>GPGSKPFTLPILTIGELSNSRFPAPIDELYTSPNEGLVVQPQNGRSTLDGELLGTTQLVPSNICSLRGRINAHLPDNQHRWNMQVTNANGTPFDPTEDVPAPLGTPDFLANIYGVTSQRNPDNTCRAHDGILATWSPKFTPKLGSVVLGTWEDRDFDINQPTRFTPVGLYDTDHFNQWALPNYSGALTLNMNLAPSVAPLFPGEQLLFFRSHIPLKGGTSNGAIDCLLPQEWVQHFYQESAPSSTDVALIRYTNPDTGRVLFEAKLHRQGFITVANSGSRPIVVPPNGYFRFDSWVNQFYSLAPM[2x]

The norovirus genome contains three open reading frames (ORF1 to 3), where ORF1 encodes the nonstructural proteins, ORF2 encodes the capsid protein (VP1), and ORF3 encodes a minor structural protein (VP2). The S domain forms a scaffold surrounding the viral RNA, whereas the P domain contains the determinants of strain diversity and recognition of attachment factors. There is considerable antigenic drift among human noroviruses, and new genetic variants evolve every other year, which can result in new epidemics worldwide. It is well known that human noroviruses bind with various specificities to histo-blood group antigens (HBGAs), which are present in saliva, on the surface of epithelial cells, and in mucosal secretions. To elucidate the constraints on non-HBGA binders from a structural perspective, we determined the X-ray crystal structures of the capsid-protruding domains (P domains) of two GII.1 (HV and noro485) nonbinders and one GII.2 (SMV) HBGA nonbinder.

HV was the first GII.1 virus detected in 1977 (15), noro485 (GII.1) was discovered in ~2005 (16), and SMV (GII.2) was identified in 1982 (17). HV, noro485, and SMV P domains diffracted to 1.86, 1.50, and 1.60 Å resolutions, respectively. The equivalent residues in the HV P domain were Cys345, Arg346, Asp375, and Gly438; in noro485, they were Cys345, Arg346, Asp375, and Gly438; and in SMV, they were Asn352, Arg353, Asp382, and Gly445. In the noro485 and SMV structures, Asp375 and Asp382, respectively, were pointing ~180° away from the fucose, whereas in the HV structure, Asp375 was missing because of the lack of electron density. Additionally, in the noro485 P domain structure, the polypeptide backbone of the loop hosting Asp375 (termed loop A) superimposed poorly onto the corresponding GII. Moreover, a neighboring loop (termed loop B) may have influenced the orientation and stability of loop A. For example, in noro485, loop B was oriented differently from that of GII. However, our new data indicate that Asp375 in HV, Asp375 in noro485, and Asp382 in SMV are unable to participate in the stabilization of the fucose moiety of HBGAs because of their flexibility or suboptimal orientation.>[2x]MNLLFQSYLDNVGVQIVRQMRSGERF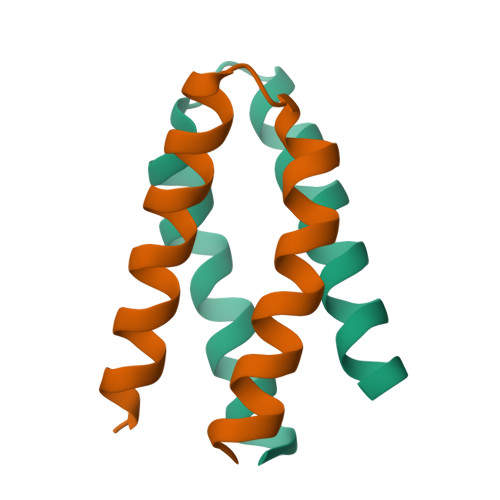LKIWSQTVEEIVSYVTVNF>[2x]MMGRGKLILIEGLDRTGKTTQCNILYKKLQPNCKLLKFPERSTRIGGLINEYLTDDSFQLSDQAIHLLFSANRWEIVDKIKKDLLEGKNIVMDRYVYSGV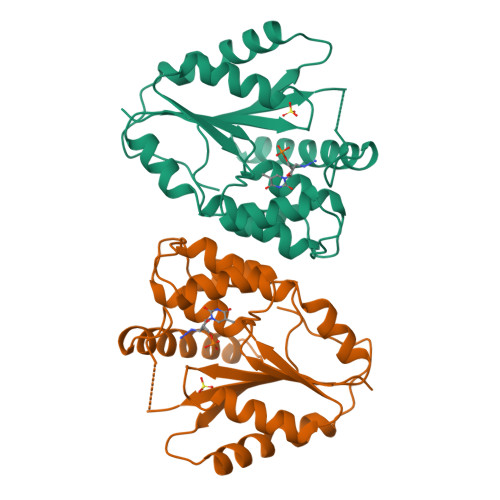AYSAAKGTNGMDLDWCLQPDVGLLKPDLTLFLSTQDVDNNAEKSGFGDERYETVKFQEKVKQTFMKLLDKEIRKGDESITIVDVTNKGIQEVEALIWQIVEPVLSTHIDHDKFSFF> MPVITVNTNVAEKSIPVFFQAALTNMMTKALQKPKEVMFVDLRSGANIMMGGDRNPCVFATVECIGRLNPTSNLAMARDMEDMFIEHLNVRRERIVIRFIP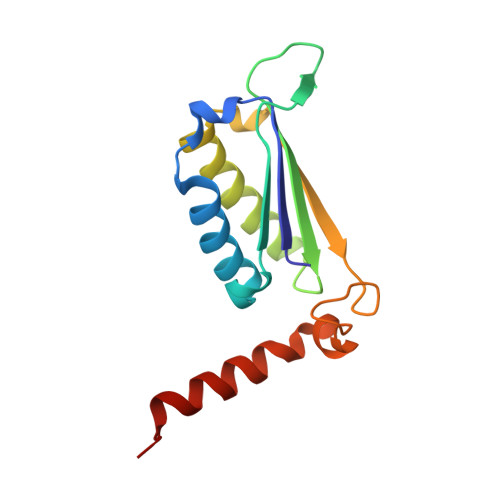VPALFCSFNGALHDVSIERDEDIISQAIAEYLHHHAHH> GHMDIAEPAELDADELKRVLEALLLVIDTPVTADALAAATEQPVYRVAAKLQLMADELTGRDSGIDLRHTSEGWRMYTRARFAPYVEKLLLDGARTKLTRAALETLAVVAYRQPVTRARVSAVRGVNVDAVMRTLLARGLITEVGTDADTGAVTFA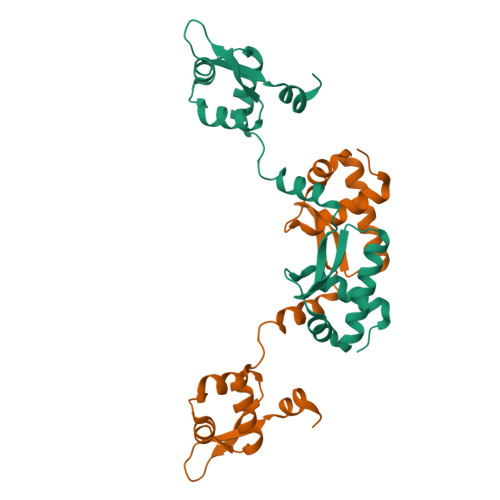TTELFLERLGLTSLSELPDIAPLLPDVDTIDDLSESLDSEPRFIKLTGELASEQTLSFDVDRD> KSIEDRIKNFFQSGGKYTELEV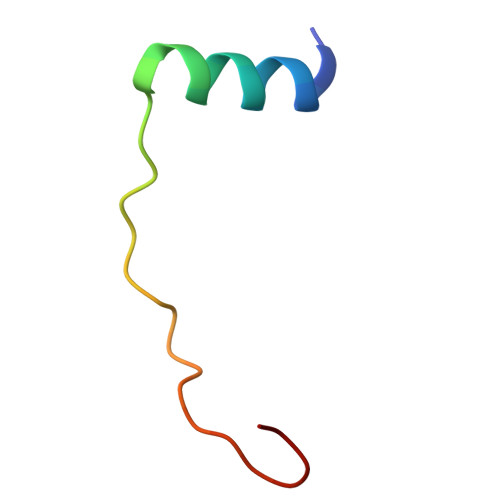DWEERVGREI>MMISEIRQELTDHIIPFWNKLRDDENGGFYGYLSYGLELDKKADKGVILHSRILWFYSNAYMTLGGDELLDNAKHAYEFIKNNCIDYEYGGVYWMMDFEGKPADTMKHTYNIAFAIYALSSYYRASGDKEALALAYRLFEDIEKNTLYEYGYREAFDRQWRLVDNEALSENGLKADKTMNAILHLIEAYTELYKADGNEKVADRLKFQLGQMRDIVYTPDTNALKVFFDTAFNLVGDIHSYGHDIEATWLMDRACDVLGDEDLKKQFAEMDLKISHNIQD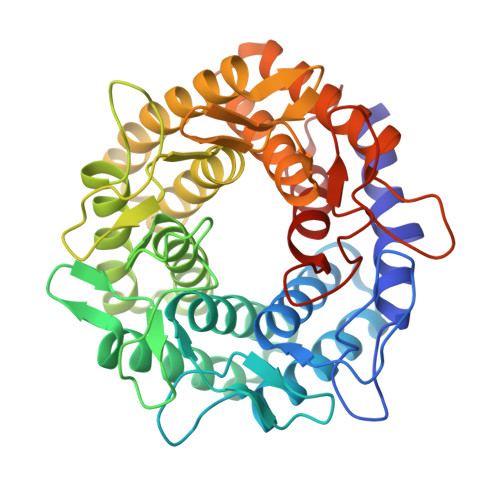IALEDGALNNERDKNEIDKTRVWWVQAEAVVGFINAYQHSGDEKFLESAKSVWENIKEYIIDKREGGEWYSEVTFDHTPHDYKETVGPWKCPYHNGRMCMEVITRGVDI[3x]(1S)-2-oxo-1-phenyl-2-[(1,3,4-trioxo-1,2,3,4-tetrahydroisoquinolin-5-yl)amino]ethyl acetate | 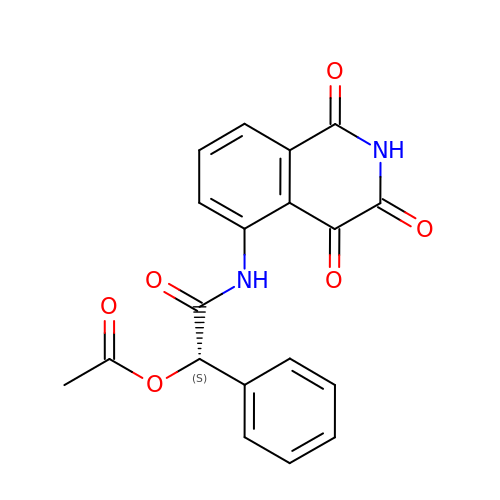C19 H14 N2 O6 | NKBDSMREMMRFSI-INIZCTEOSA-N> GKENEENIQCGENFMDIECFMVLNPSQQLAIAVLSLTLGTFTVLENLLVLCVILHSRSLRCRPSYHFIGSLAVADLLGSVIFVYSFIDFHVFHRKDSRNVFLFKLGGVTASFTASVGSLFLAAIDRYISIHRPLAYKRIVTRPKAVVAFCLMWTIAIVIAVLPLLGWNCEKLQSVCSDIFPHIDETYLMFWIGVTSVLLLFIVYAYMYILWKAGIDCSFWNESYLTGSRDERKKSLLSKFGMDEGVTFMFIGRFDRGQKGVDVLLKAIEILSSKKEFQEMRFIIIGKGDPELEGWARSLEEKHGNVKVITEMLSREFVRELYGSVDFVIIPSYFEPFGLVALEAMCLGAIPIASAVGGLRDIITNETGILVKAGDPGELANAILKALELSRSDLSKFRENCKKRAMSFSDQARMDIRLAKTLVLILVVLIICWGPLLAIMVYDVFGKMNKLIKTVFAFCSMLCLLNSTVNPIIYALRSKDLRHAFRSMFPSCEGTAQPHHHHHHHHHH

The endocannabinoid signaling system in mammals is comprised of the endogenous lipid messengers anandamide and 2-AG and two homologous GPCRs, CB1 located in the nervous system and periphery and CB2 expressed primarily in immune cells. CB1 is the most abundant GPCR in the central nervous system (CNS) and regulates diverse brain functions and behaviors, modulating neurotransmitter release and neuronal excitation through pre-synaptic activation of Gi/o, GIRK channels, and arrestin/MAP kinase signaling. To gain further insight into the molecular mechanisms of cannabinoid system modulators and enable structure-based ligand design, we sought to crystallize and solve the atomic structure of the human CB1 receptor. CB1's orthosteric binding pocket is highly hydrophobic, as expected for a lipid-activated receptor.

To promote LCP crystallization, we replaced the third intracellular loop (ICL3) of CB1 with the thermostable PGS domain, which recently proved essential in solving crystal structures of the human orexin receptors. We incorporated the point mutation T210A, which was previously shown to stabilize the inactive conformation of CB1 and increase thermostability. Finally, we truncated CB1T210A-PGS by eliminating the first 89 N-terminal residues and the C-terminus after residue 421. After purifying this construct from Sf9 insect cells, we obtained LCP microcrystals that diffracted to 2.6 Å resolution, solved the structure by molecular replacement, and refined the structure to Rfree 0.23. At the extracellular surface, the second extracellular loop (ECL2) and membrane-proximal N-terminal region preceding transmembrane domain 1 (TM1) form a lid over the orthosteric pocket, which almost completely shields taranabant from solvent. Taranabant makes multiple contacts to both TM1 and TM7 and fills the orthosteric pocket directly inside the TM1-TM7 opening, potentially acting as a ‘plug’ to block endocannabinoid entrance. Taranabant adopts a conformation in which the chlorophenyl moiety extends toward TM5, the cyanophenyl buries deeper into the 7TM bundle, and the trifluoromethylpyridine projects into the putative access channel between TM1 and TM7. Of the 24 residues within 4 Å of the ligand, there are only three polar sidechains – D104 whose acidic sidechain points toward the extracellular space, S1231.39 near the access channel that forms a polar contact with taranabant's trifluoromethyl group, and S3837.39 that has been implicated in agonist binding. In contrast, a large number of hydrophobic residues (including 6 Phe, 3 Met, 2 Trp, 3 Leu, and 3 Ile sidechains) line the orthosteric pocket and make a variety of hydrophobic contacts to taranabant, burying 1109 Å2 of surface area. The major divergence between CB1 and CB2 within the subset of binding residues lies in the membrane-proximal N-terminal region, where F102, M103, D104, I105, and F108 make van der Waals contacts to taranabant.>MAETEIHTFDDIPMPKLADPLLIYTPANEIFDIASCSAKDIGFAIAHAQIPPGGGPMPHIHYFINEWFWTPEGGIELFHSTKQYPNMDELPVVGGAGRGDLYSIQSEPKQLIYSPNHYMHGFVNPTDKTLPIVFVWMRNEVAPDFPYHDGGMREYFQAVGPRITDLNNLPELTNAQRAAFASEAPKYGINQSSYFMEYVNTISDKLPAQIAKLKNDKDLE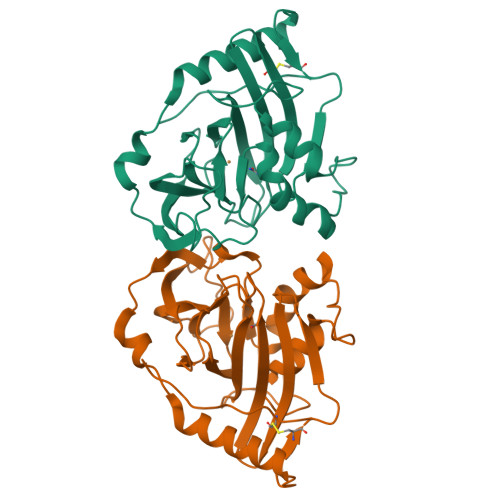RMVEVIEAFNRGDKSVTCS[4x]> GLPVMNTP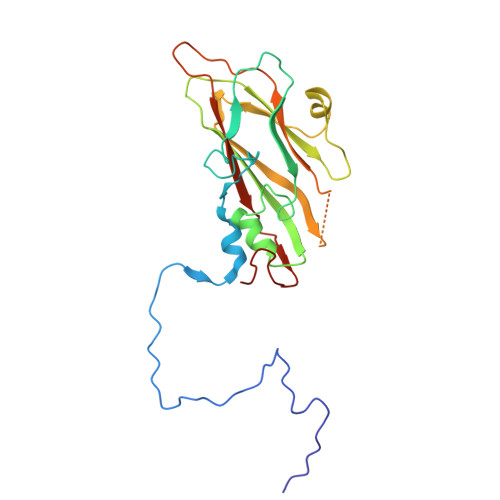GSNQFLTSDDYQSPTAMPQFDVTPEMNIPGEVKNLMEIAEVDSVVPVNNVNENVNSLEAYRIPVHSVTETGAQVFGFTLQPGADTVMERTLLGEILNYYANWSGSIKLTFMYCGSAMATGKFLLAYSPPGAGVPKNRREAMLGTHIIWDIGLQSSCVLCVPWISQTHYRFVSKDSYTDAGFITCWYQTSIVVPAEVQNQSVILCFVSACNDFSVRLLRDSPFVRQT(2R)-2-(7-carbamoyl-1H-benzimidazol-2-yl)-2-methylpyrrolidinium | C13 H16 N4 O | 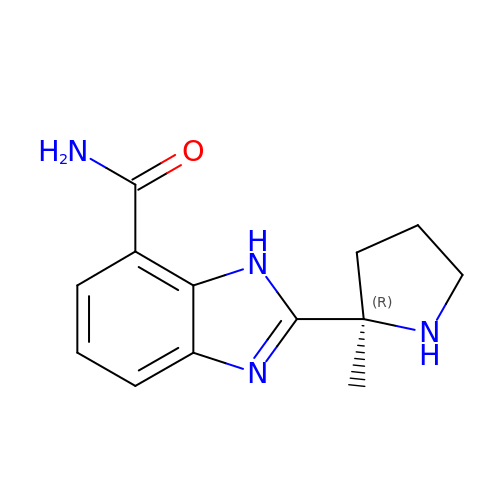JNAHVYVRKWKWKQ-CYBMUJFWSA-N> TAVEAVHAWRNALTGAPLNLTPEQVVAIASHDGGKQALETVQRLLPVLCQAHGLTPQQVVAIASHDGGKQALETVQRLLPVLCQAHGLTPEQVVAIASHDGGKQALETVQALLPVLCQAHGL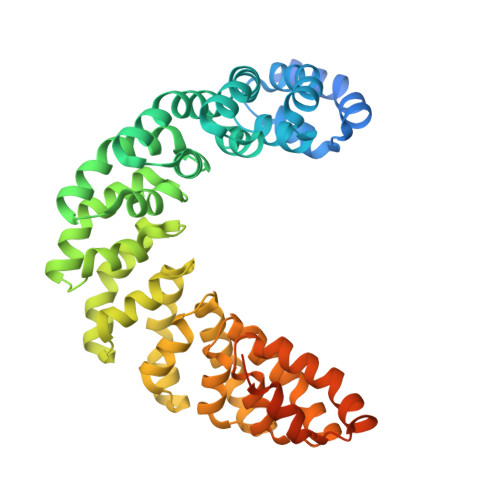TPEQVVAIASNGGGKQALETVQRLLPVLCQAHGLTPQQVVAIASNGGGKQALETVQRLLPVLCQAHGLTPQQVVAIASNGGGKQALETVQRLLPVLCQAHGLTPQQVVAIASNSGGKQALETVQRLLPVLCQAHGLTPQQVVAIASNGGGKQALETVQRLLPVLCQAHGLTPQQVVAIASHDGGKQALETVQRLLPVLCQAHGLTPEQVVAIASNGGGKQALETVQRLLPVLCQAHGLTPEQVVAIASHDGGKQALETVQRLLPVLCQAHGLTPQQVVAIASNGGGRPALESIVAQLSRPDPALAALTNDHLLEHHHHHH>[2x]MSGA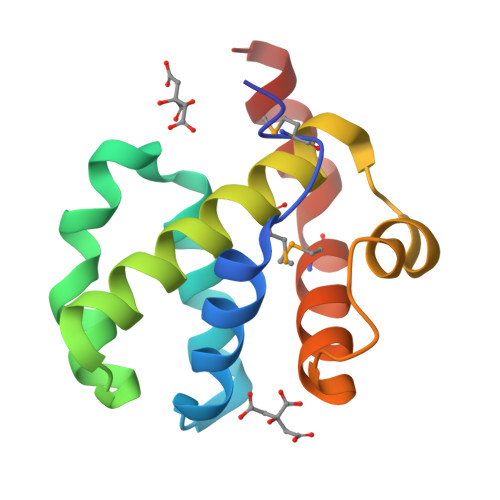MAALTAEHFAALQSLLKASSKDVVRQLCQESFSSSALGLKKLLDVTCSSLSVTQEEAEELLQALHRMTRLVAFRDLSSAEAILALFPENFHQNLKNLLTKIMLEHVSTWRTEAQANQ> MAYRKRGARRETNLKQDDRMQEKEENKNVNTNSENKNATKPQLSEKVLSQKEEVITDNQEEIKIADEVKKSNKEESKQLLEVLKTKEEHQKEVQYEILQKTIPTFEPKESILKKLEDIKPEQVKKQTKLFRIFEPRQLPVYRANGEKELRNRWYWKLKRDTLPDGDYDVREYFLNLYDQVLTEMPDYLLLKDMAVENKNSRDAGKVVDSETAAICDAIFQDEETEGVVRRFIAEMRQRVQADRNVVNYPSILHPIDHAFNEYFLQHQLVEPLNNDIIFNYIPERIRNDVNYILNMDRNLPSTARYIRPNLLQDRLNLHDNFESLWDTITTSNYILARSVVPDLKELVSTEAQIQKMSQDLQLEALTIQSETQFLTGINSQAANDCFKTLIAAMLSQRTMSLDFVTTNYMSLISGMWLLTVVPNDMFIRESLVACQLAIINTIIYPAFGMQRMHYRN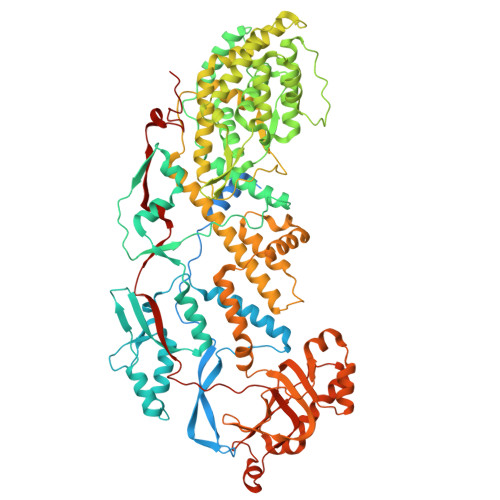GDPQTPFQIAEQQIQNFQVANWLHFVNNNQFRQVVIDGVLNQVLNDNIRNGHVVNQLMEALMQLSRQQFPTMPVDYKRSIQRGILLLSNRLGQLVDLTRLLAYNYETLMACITMNMQHVQTLTTEKLQLTSVTSLCMLIGNATVIPSPQTLFHYYNVNVNFHSNYNERINDAVAIITAANRLNLYQKKMKSIVEDFLKRLQIFDISRVPDDQMYRLRDRLRLLPVEIRRLDIFNLILMNMEQIERASDKIAQGVIIAYRDMQLERDEMYGYVNIARNLDGFQQINLEELMRTGDYAQITNMLLNNQPVALVGALPFITDSSVISLVAKLDATVFAQIVKLRKVDTLKPILYKINSDSNDFYLVANYDWVPTSTTKVYKQIPQQFDFRASMHMLTSNLTFTVYSDLLAFVSADTVEPINAVAFDNMRIMNEL>MMKIAILDDYQNVVRGLNAFQCLQGHDVTVFNDSVSDETVLIERLKPFEALVLIRERTPITENLLAHLPNLKLISQTGKVSNHIDVPLCERYGVTVLEGIGSPVAPAELCWSLILAASRHLPSYIEQLHAGHWQQNGGLGLGRTLSGRTLGIWGLGKIGQRIAQFGHVFGMPILVWGSEASRQKALELGYQAAADKAEFFAKADVLSLHLRLNDATRGIVTKQDLLAMKPDSLFVNTSRAELVESGALYSVMQANPMRQAAVDVYENEPALPNNEPLLSLPNVLCAPHLGYVEKNSYEIYFQAAFENVVKFAHSAAK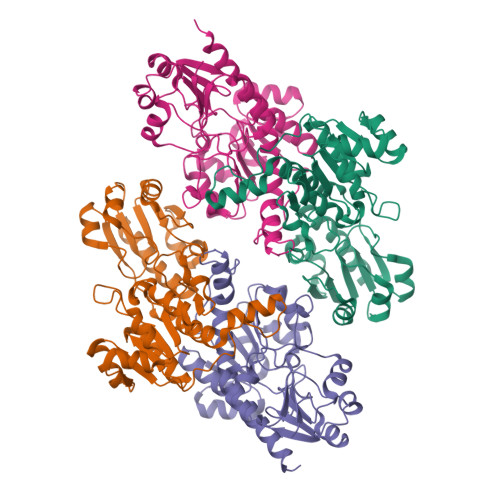ASLSDKALEHHHHHH[4x]> MSSERTFIAVKPDGVQRGLAGEVICRFERKGYKLVALKMLQPTTEQAEGHYKDLSSKPFFPALVKYFSSGPIVCMVWEGKNVVKGGRMLLGATNPADSHPGTIRGDFAVDMGRNVCHGSDS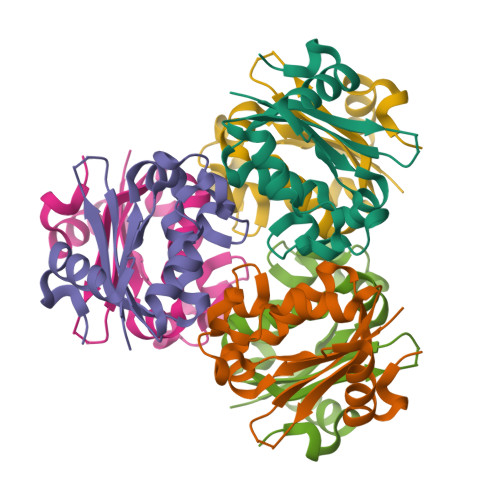VESAEREIAFWFKADELACWTSHSVSQIYE> GPLGSGSGDDLFAGLKKKKKKSKSVSADAEAEKEPTDDIAEALGELSLKKKKKKTKDSSVDAFEKEL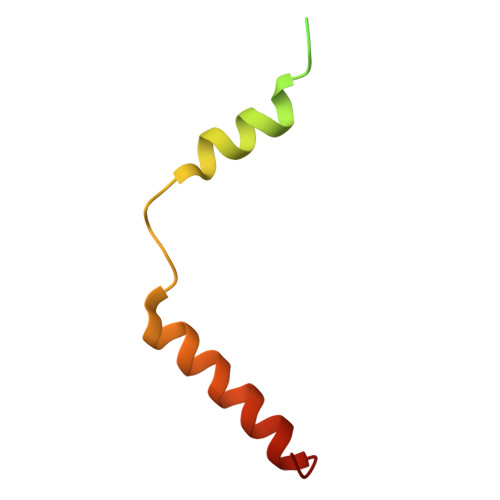AKAGLD> MIQGVIQKIAGPAVIAKGMLGARMYDISKVGEEGLVGEIIRLDGDTAFVQVYEDTSGLKVGEPVVSTGLPLAVELGPGMLNGIYDGIQRPLERIREKTGIYITRGVVVHALDREKKWAWTPMVKPGDEVRGGMVLGTVPEFGFTHKILVPPDVRGRVKEVKPAGEYTVEEPVVVLEDGTELKMYHTWPVRRARPVQRKLDPNTPFLTGMRILDVLFPVAMGGTAAIPGPFGSGKSVTQQSLAKWSNADVVVYVGSGERGNEMTDVLVEFPELTDPKTGGPLMHRTVLIAN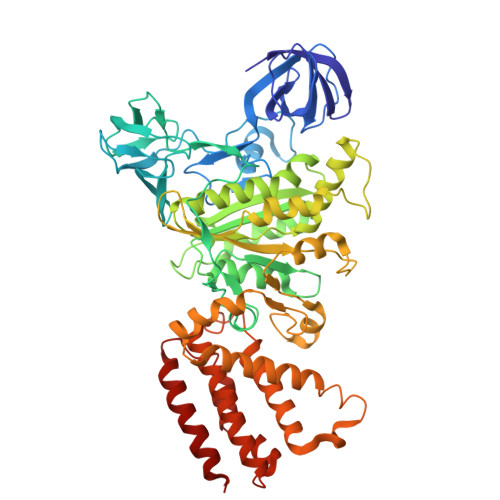TSNMPVAAREASIYVGVTIAEYFRDQGFSVALMADSTSRWAEALREISSRLEEMPAEEGYPPYLAARLAAFYERAGKVITLGGEEGAVTIVGAVSPPGGDMSEPVTQSTLRIVGAFWRLDASLAFRRHFPAINWNGSYSLFTSALDPWYRENVAEDYPELRDAISELLQREAGLQEIVQLVGPDALQDAERLVIEVGRIIREDFLQQNAYHEVDAYSSMKKAYGIMKMILAFYKEAEAAIKRGVSIDEILQLPVLERIGRARYVSEEEFPAYFEEAMKEIQGAFKALA>MASKKVHQINVKGFFDMDVMEVTEQTKEAEYTYDFKEILSEFNGKNVSITVKEENELPVKGVEMAGDPLEH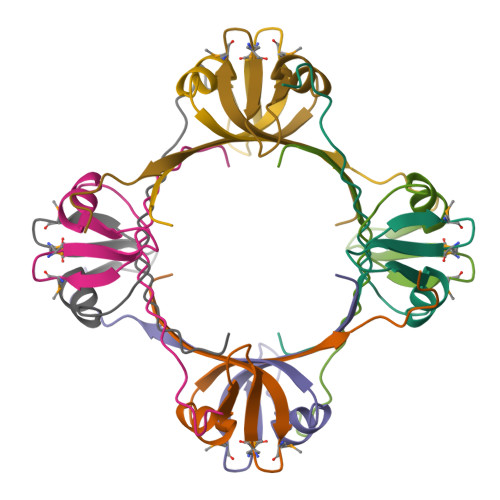HHHHH[4x]5-CHLORO-2-(2-CHLORO-4-NITROPHENOXY)PHENOL | C12 H7 Cl2 N 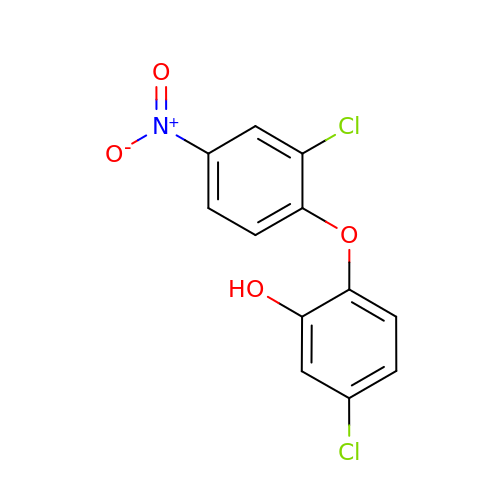O4 | DEDBMNCDHFNYKX-UHFFFAOYSA-N>[3x]SGQDLVPAAVEQAVPIQPVAGAALAAPAAGQINQIDPWIFQNFVQCPLGEFSISPRNTPGEILFDLALGPGLNPYLAHLSAMYTGWVGNMEVQLVLAGNAFTAGKVVVALVPPYFPKGSLTTAQITCFPHVMCDVRTLEPIQLPLLDVRRVLWHATQDQEESMRLVCMLYTPLRTNSPGDESFVVSGRLLSKPAADFNFVYLTPPIERTIYRMVDLPVIQPRLCTHARWPAPVYGLLVDPSLPSNPQWQNGRVHVDGTLLGTTPISGSWVSCFAAEAAYEFQSGTGEVATFTLIEQDGSAYVPGDRAAPLGYPDFSGQLE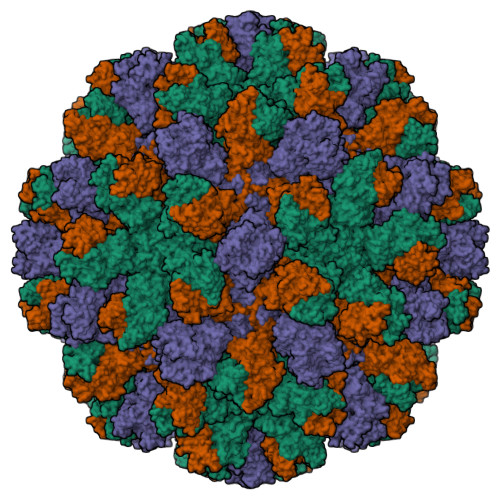IEVQTETTKTGDKLKVTTFEMILGPTTNADQAPYQGRVFASVTAAASLDLVDGRVRAVPRSIYGFQDTIPEYNDGLLVPLAPPIGPFLPGEVLLRFRTYMRQIDTADAAAEAIDCALPQEFVSWFASNAFTVQSEALLLRYRNTLTGQLLFECKLYNEGYIALSYSGSGPLTFPTDGIFEVVSWVPRLYQLASVGS> EDENVKKFIKEFEDTKIMPVRKGTKTTRTEKFYLVFTEWVKLLQRVENNDVITTVFIKQLVEKGVISDTDNLLTFVKSSLELSVSSFKESDPTDEVFIAIDALGSLIIKLLILQDFKDDTRRDYINAIFSVIVLVFAKDHSQEGTTFNERPYFRLFSNILYEWATIRTHNFVRISDSSTRQELIEFDSVFYNTFSGYLHALQPFAFPGFSFAWVTLLSHRMLLPIMLRLPNKIGWEKLMLLIIDLFKFLDQYTS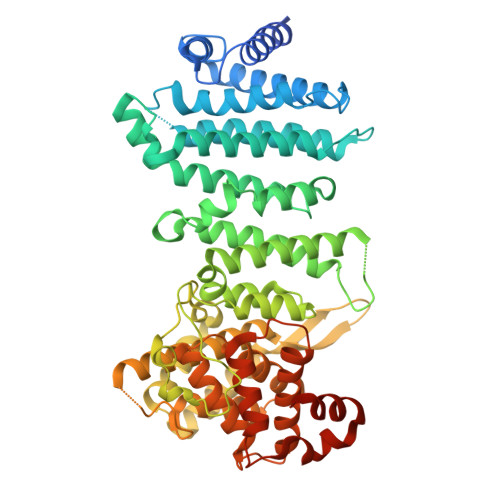KHAVSDAVSVVYKGTLRIILGISNDMPSFLIENHYELMNNLPPTYFQLKNVILSAIPKNMTVPNPYDVDLNMEDIPACKELPEVFFDPVIDLHSLKKPVDNYLRIPSNSLLRTILSAIYKDTYDIKKGVGYDFLSVDSKLIRAIVLHVGIEAGIEYKRTSSNAVFNTKSSYYTLLFNLIQNGSIEMKYQIILSIVEQLRYPNIHTYWFSFVLMNMFKSDEWNDQKLEVQEIILRNFLKRIIVNKPHTWGVSVFFTQLINNNDINLLDLPFVQSVPEIKLILQQLVKYSKKYTTSEQDDQ> MAGNQRQGVAFIRVNGMELESMEGASFTPSGITREEVTGSRVYGWKGKPRAAKVECKIPGGGPIGLDEIIDWENITVEFQAD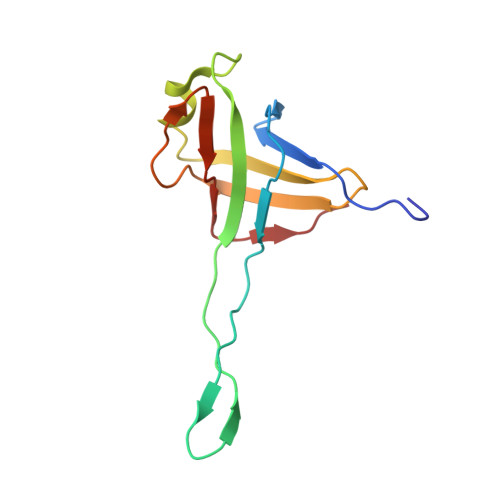TGETWMLANAWQADEPKNDGGEISLVLMAKQSKRIA> KILH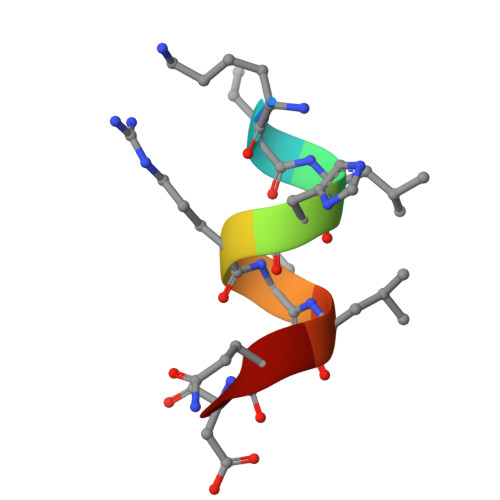RLLQD>MGHHHHHHGQQDVHGPFQGQRQNEFDLMFVKEIFKNHNSNVVLSPFSVKILLTLIYEASDTSFGNAVSNTKRELSSVIQNDNIDHTRSYYKQLLESAQQDNKDYDLNIATNFFVDDFIEVINKYQQIANTHYHAMLEKVSYSNPTQTAATINNWVSEHTNGRLREIVTPDSLEGAVITLVNVIYFCGLWTYPFPEVANNVKPFYGTRGKPTNAQYMEQNGQFYYDNSADLGAQILRLPYRGNKLAMYFILPNPDNTVNQVLDRINSASLHQALWYMEENEVNVTLPKFKFDFSEQLNEPLQQVGIREIFSQNASLPLLARGRGARDEVRVSRIFQKAGITINELGSCAYAATE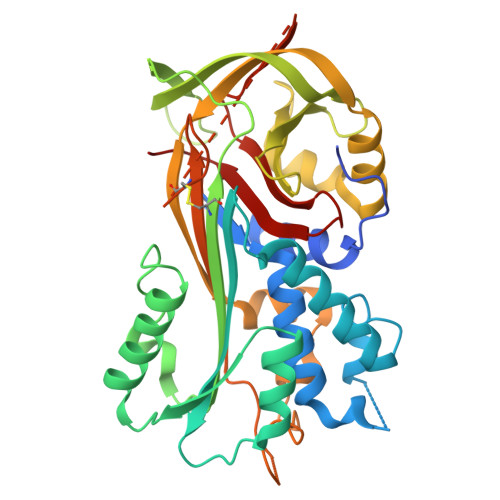IQLVNKFGGDGVQIFNANRPFIFFIEDETLGTMLFAGKIENPVF[12x]> GSPESFPDAHMRMILRKPPGQRTVDDLEIIYDELLHIKALSHLSTTVKRELAGVLIFESHAKGGTVLFNQGEEGTSWYIILKGSVNVVIYGKGVVCTLHEGDDFGQLALVNDAPRAASIVLREDNCHFLRVDKEDFNRILRDVEANTVRLKEHDQDVLVLEKVPAGNRAANQGNSQPQQKYTVMSGTPEKILEHFLETIRLEPSLNEATDSVLNDFVMMHCVFMPNTQLCPALVAHYHAQPSQGTEQERMDYALNNKRRVIRLVLQWAAMYGDLLQEDDVAMAFLEEFYVSVSDDARMMAAFKEQLPELEKIVKQISEDAKAPQKKHKVLLQQFNTGDERAQKRQPIRGSDEVLFK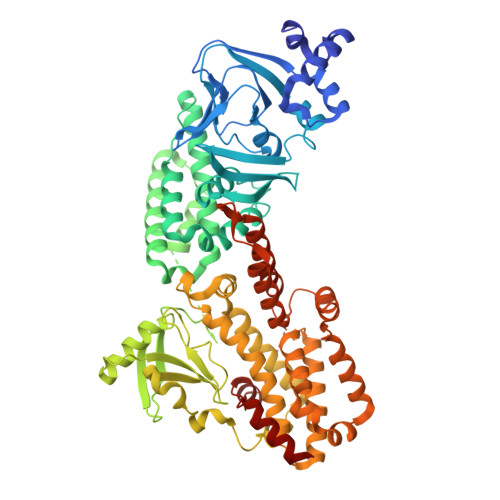VYCIDHTYTTIRVPVAASVKEVISAVADKLGSGEGLIIVKMNSGGEKVVLKSNDVSVFTTLTINGRLFACPREQFDSLTPLPEQEGPTTGTVGTFELMSSKDLAYQMTTYDWELFNCVHELELIYHTFGRHNFKKTTANLDLFLRRFNEIQFWVVTEVCLCSQLSKRVQLLKKFIKIAAHCKEYKNLNSFFAIVMGLSNVAVSRLALTWEKLPSKFKKFYAEFESLMDPSRNHRAYRLTAAKLEPPLIPFMPLLIKDMTFTHEGNKTFIDNLVNFEKMRMIANTARTVRYYRSQPFNPDAAQANKNHQDVRSYVRQLNVIDNQRTLSQMSHRLEPRRP>[2x]MDWVIPPISLPENEKGPFPKNLVQIKSNKDKEGKVFYSITGQGADTPPVGVFIIERETGWLKVTEPLDRERIATYTLFSHAVSSNGNAVEDPM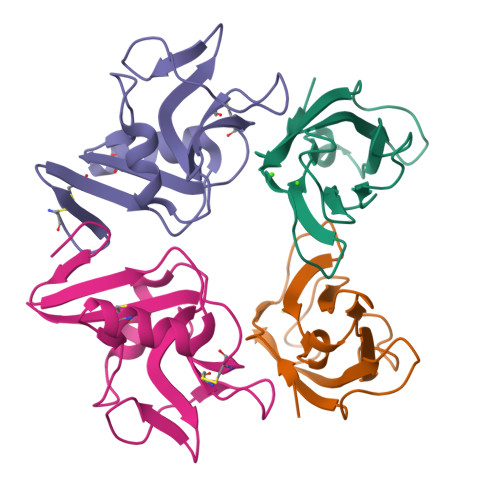EILITVTD;>CPILWTRNGSHCYYFSMEKKDWNSSLKFCADKGSHLLTFPDNQGVKLFGEYLGQDFYWIGLRNIDGWRWEGGPALSLRILTNSLIQRCGAIHRNGLQASSCEVALQWICKKVLY[2x]beta-Saxitoxinol | C10 H17 N7 O3 | 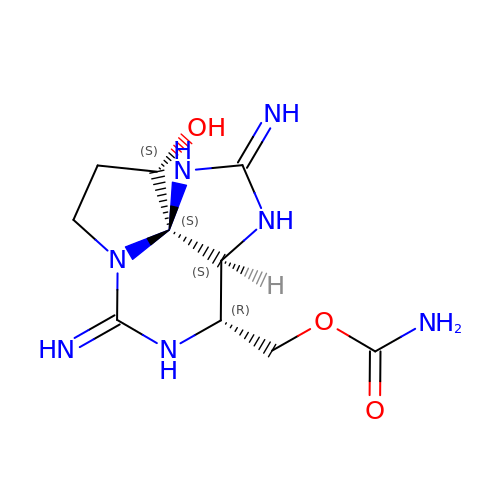NILHUXIFTLLDPJ-AVGUDYQDSA-N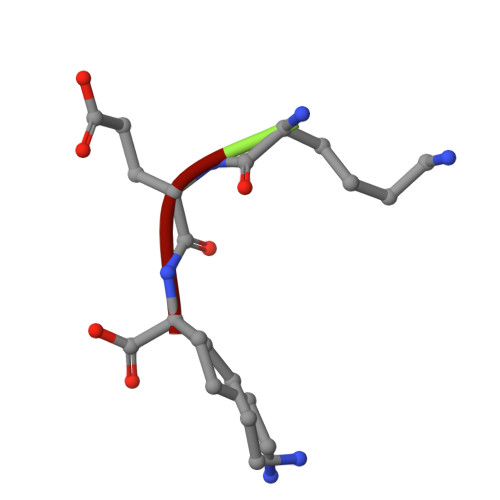> KEK Calcium/Calmodulin (Ca2+/CaM)-dependent serine/threonine kinases (CaMKs) constitute a family of 81 proteins in the human proteome that play a central role in cellular signaling by transmitting Ca2+ signals. Kinases in this protein family are activated through binding of Ca2+/CaM to regulatory regions that either flank the catalytic domain or are located in regulatory molecules. CaMKII proteins form large oligomeric structures. The N-terminal kinase domain is tethered via an autoinhibitory helix and a calmodulin binding site to a C-terminal oligomerization domain that organizes the enzyme into ring-shaped oligomers.

The discrepancy between the dodecameric (12-mer) structures determined by electron microscopy and the tetradecameric (14-mer) assembly revealed by the crystal structure of the isolated oligomerization domain of the C. elegans orthologue prompted us to crystallize the oligomerizaton domains of human CaMKII isozymes. Here we present the oligomerization domains of the human γ and δ isozymes that were refined at 2.7 and 2.8 Å resolution, respectively. While isolated domains of the δ isozyme were tetradecameric, the CaMKIIγ oligomerization domain crystallized in its dodecameric state, thus providing a model for the oligomerization state observed in full-length CaMKIIs. The oligomerization domain formed a hexameric structure with a diameter of 120 Å and a height of 60 Å surrounding a central cavity of only 17 Å. Thus, the main consequence of the insertion of an additional subunit per ring in the tetradecameric assembly is a considerable widening of the central cavity, to about 33 Å. Each oligomerization domain in the ring also contains a deep cavity that has been suggested to represent a peptide binding site, based on structural homology with peptide-binding domains present in nuclear transport factors and scytalone dehydratase. In support of this hypothesis is the fact that a glycine or an acetate molecule, respectively, originating from the crystallization solution were partially occupying this putative binding site in the structures of the CaMKIIγ and CaMKIIδ oligomerization domains. We used the structures of the dodecameric oligomerization domain, the CaMKIIδ/Ca2+/CaM complex and the structures of the inactive catalytic domains, to construct models for the full-length enzyme.

>[6x]SMTEDEDLKVRKQEIIKITEQLIEAINNGDFEAYTKICDPGLTSFEPEALGNLVEGMDFHKFYFENLLSKNSKPIHTTILNPHVHVIGEDAACIAYIRLTQYIDGQGRPRTSQSEETRVWHRRDGKWLNVHYHCSGAPAAPRQ5'-O-[(3-Indolyl)-1-Ethyl]Carbamoyl 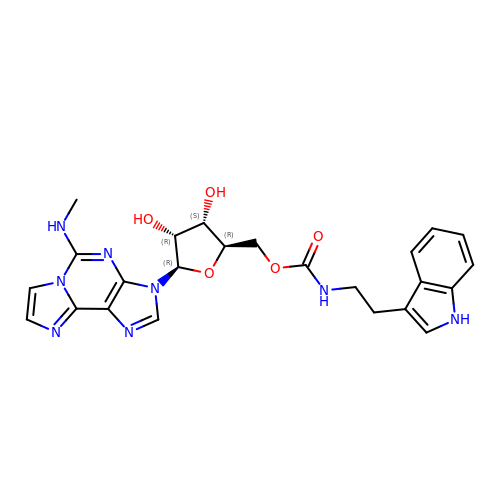N2-methyl-2-aminoethenoadenosine | C24 H26 N8 O5 | CBOHRQLNXCBGQM-WGQQHEPDSA-N> SNAMRFTLLAFALAVALPAVHASAAEAPLPQLRAYTVDASWLQPMAPLQVADHTWQIGTEDLTALLVQTAEGAVLLDGGMPQMAGHLLDNMKLRGVAPQDLRLILLSHAHADHAGPVAELKRRTGAHVAANAETAVLLARGGSNDLHFGDGITYPPASADRIIMDGEVVTVGGIAFTAHFMPGHTPG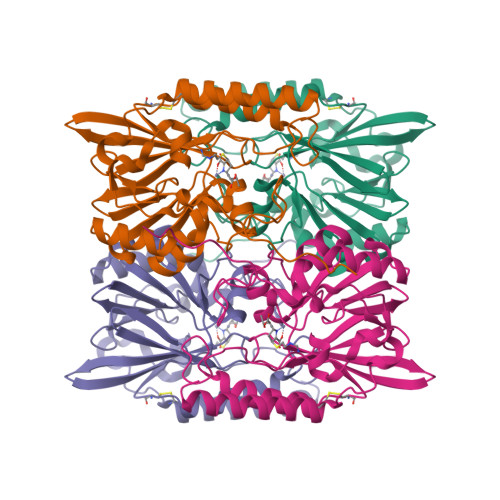STAWTWTDTRDGKPVRIAYADSLSAPGYQLKGNPRYPRLIEDYKRSFATVRALPCDLLLTPHPGASNWNYAVGSKASAEALTCNAYADAAEKKFDAQLARETAGTR> MSQLVLILGDQLSPSIAALDGVDKKQDTIVLCEVMAEASYVGHHKKKIAFIFSAMRHFAEELRGEGYRVRYTRIDDADNAGSFTGEVKRAIDDLTPSRICVTEPGEWRVRSEMDGFAGAFGIQVDIRSDRRFLSSHGEFRNWAAGRKSLTMEYFYREMRRKTGLLMNGEQPVGGRWNFDAENRQPARPDLLRPKHPVFAPDKITKEVIDTVERLFPDNFGKLENFGFAVTRTDAERALSAFIDDFLCNFGATQDAMLQDDPNLNHSLLSFYINCGLLDALDVCKAAERAYHEGGAPLNAVEGFIRQIIGWREYMRGIYWLAGPDYVDSNFFENDRSLPVFYWTGKTHMNCMAKVITETIENAYAHHIQRLMITGNFALLAGIDPKAVHRWYLEVYADAYEWVELPNVIGMS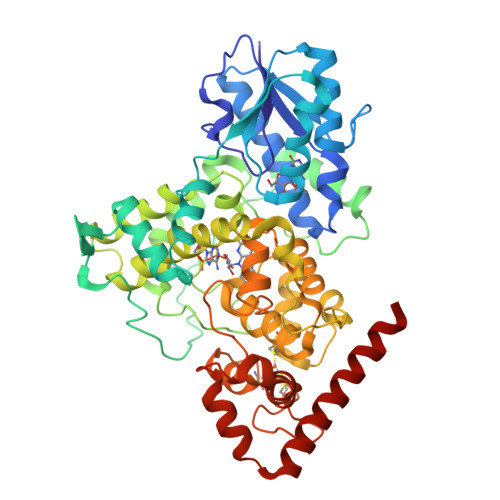QFADGGFLGTKPYAASGNYINRMSDYCDTCRYDPKERLGDNACPFNALYWDFLARNREKLKSNHRLAQPYATWARMSEDVRHDLRAKAAAFLRKLDAAALEHHHHHH>[2x]MKKIKPHGPLPSQTQLAYLGDELAAFIHFGPNTFYDQEWGTGQ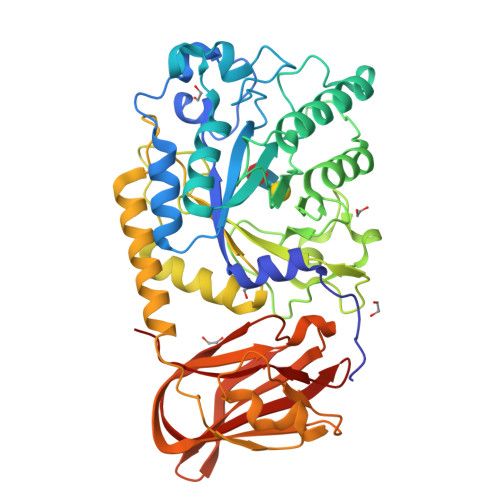EDPERFNPSQLDAREWVRVLKETGFKKLILVVKHHDGFVLYPTAHTDYSVKVSPWRRGKGDLLLEVSQAATEFDMDMGVYLSPWDAHSPLYHVDREADYNAYYLAQLKEILSNPNYGNAGKFAEVWMNGARGEGAQKVNYEFEKWFETIRDLQGDCLIFSTEGTSIRWIGNQRGYAGDPLWQKVNPDKLGTEAELNYLQHGDPSGTIFSIGEADVSIRPGWFYHEDQDPKSLEELVEIYFHSVGRGTPLLLNIPPNQAGLFDAKDIERLYEFATYRNELYKEDLALGAEVSGPALSADFACRHLTDGLETSSWASDADLPIQLELDLGSPKTFDVIELREDLKLGQRIAAFHVQVEVDGVWQEFGSGHTVGYKRLLRGAVVEAQKIRVVITESQALPLLTKISLYKTPG>[4x]ADPGKSCPSVCRCDAGFIYCNDRFLTSIPTGIPEDATTLYLQNNQINNAGIPSDLKNLLKVERIYLYH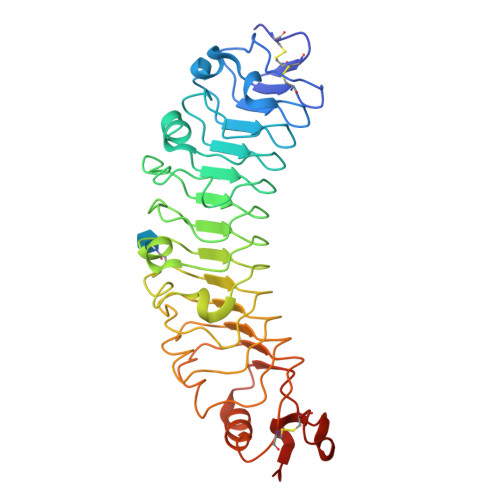NSLDEFPTNLPKYVKELHLQENNIRTITYDSLSKIPYLEELHLDDNSVSAVSIEEGAFRDSNYLRLLFLSRNHLSTIPWGLPRTIEELRLDDNRISTISSPSLQGLTSLKRLVLDGNLLNNHGLGDKVFFNLVNLTELSLVRNSLTAAPVNLPGTNLRKLYLQDNHINRVPPNAFSYLRQLYRLDMSNNNLSNLPQGIFDDLDNITQLILRNNPWYCGCKMKWVRDWLQSLPVKVNVRGLMCQAPEKVRGMAIKDLNAELFDCKD> DTKEQRILRYVQQNAKPGDPQSVLEAIDTYCTQKEWAMNVGDAKGQIMDAVIREYSPSLVLELGAYCGYSAVRMARLLQPGARLLTMEMNPDYAAITQQMLNFAGLQDKVTILNGASQDLIPQLKKKYDVDTLDMVFLDHWKDRYLPDTLLLEKCGL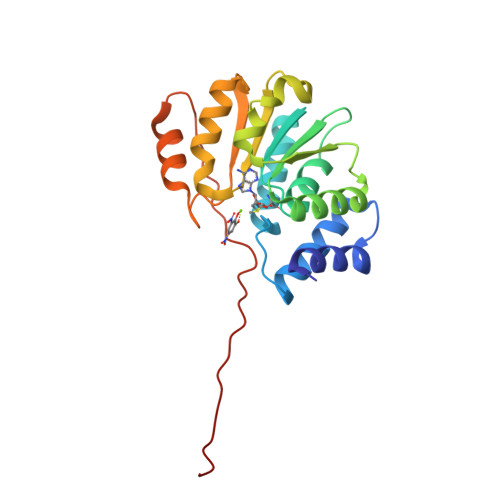LRKGTVLLADNVIVPGTPDFLAYVRGSSSFECTHYSSYLEYMKVVDGLEKAIYQGP>[2x]FNLDTEELTAFRVDSAGFGDSVVQYANSWVVVGAPQKITAANQTGGLYQCGYSTGACEPIGLQVPPEAVNMSLGLSLASTTSPSQLLACGPTVHHECGRNMYLTGLCFLLGPTQLTQRLPVSRQECPRQEQDIVFLIDGSGSISSRNFATMMNFVRAVISQFQRPSTQFSLMQFSNKFQTHFTFEEFRRSSNPLSLLASVHQLQGFTYTATAIQN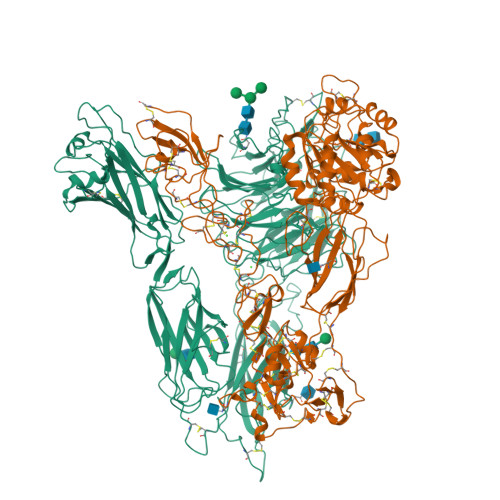VVHRLFHASYGARRDAAKILIVITDGKKEGDSLDYKDVIPMADAAGIIRYAIGVGLAFQNRNSWKELNDIASKPSQEHIFKVEDFDALKDIQNQLKEKIFAIEGTETTSSSSFELEMAQEGFSAVFTPDGPVLGAVGSFTWSGGAFLYPPNMSPTFINMSQENVDMRDSYLGYSTELALWKGVQSLVLGAPRYQHTGKAVIFTQVSRQWRMKAEVTGTQIGSYFGASLCSVDVDSDGSTDLVLIGAPHYYEQTRGGQVSVCPLPRGWRRWWCDAVLYGEQGHPWGRFGAALTVLGDVNGDKLTDVVIGAPGEEENRGAVYLFHGVLGPSISPSHSQRIAGSQLSSRLQYFGQALSGGQDLTQDGLVDLAVGARGQVLLLRTRPVLWVGVSMQFIPAEIPRSAFECREQVVSEQTLVQSNICLYIDKRSKNLLGSRDLQSSVTLDLALDPGRLSPRATFQETKNRSLSRVRVLGLKAHCENFNLLLPSCVEDSVTPITLRLNFTLVGKPLLAFRNLRPMLAADAQRYFTASLPFEKNCGADHICQDNLGISFSFPGLKSLLVGSNLELNAEVMVWNDGEDSYGTTITFSHPAGLSYRYVAEGQKQGQLRSLHLTCDSAPVGSQGTWSTSCRINHLIFRGGAQITFLATFDVSPKAVLGDRLLLTANVSSENNTPRTSKTTFQLELPVKYAVYTVVSSHEQFTKYLNFSESEEKESHVAMHRYQVNNLGQRDLPVSINFWVPVELNQEAVWMDVEVSHPQNPSLRCSSEKIAPPASDFLAHIQKNPVLDCSIAGCLRFRCDVPSFSVQEELDFTLKGNLSFGWVRQILQKKVSVVSVAEITFDTSVYSQLPGQEAFMRAQTTTVLEKYKVHGCGGLENLYFQ;>[2x]QECTKFKVSSCRECIESGPGCTWCQKLNFTGPGDPDSIRCDTRPQLLMRGCAADDIMDPTSLAETQEDHNGGQKQLSPQKVTLYLRPGQAAAFNVTFRRAKGYPIDLYYLMDLSYSMLDDLRNVKKLGGDLLRALNEITESGRIGFGSFVDKTVLPFVNTHPDKLRNPCPNKEKECQPPFAFRHVLKLTNNSNQFQTEVGKQLISGNLDAPEGGLDAMMQVAACPEEIGWRNVTRLLVFATDDGFHFAGDGKLGAILTPNDGRCHLEDNLYKRSNEFDYPSVGQLAHKLAENNIQPIFAVTSRMVKTYEKLTEIIPKSAVGELSEDSSNVVQLIKNAYNKLSSRVFLDHNALPDTLKVTYDSFCSNGVTHRNQPRGDCDGVQINVPITFQVKVTATECIQEQSFVIRALGFTDIVTVQVLPQCECRCRDQSRDRSLCHGKGFLECGICRCDTGYIGKNCECQTQGRSSQELEGSCRKDNNSIICSGLGDCVCGQCLCHTSDVPGKLIYGQYCECDTINCERYNGQVCGGPGRGLCFCGKCRCHPGFEGSACQCERTTEGCLNPRRVECSGRGRCRCNVCECHSGYQLPLCQECPGCPSPCGKYISCAECLKFEKGPFGKNCSAACPGLQLSNNPVKGRTCKERDSEGCWVAYTLEQQDGMDRYLIYVDESRECVAGPDGCGENLYFQ> GSDQPRPTVIITGASSGVGLYATK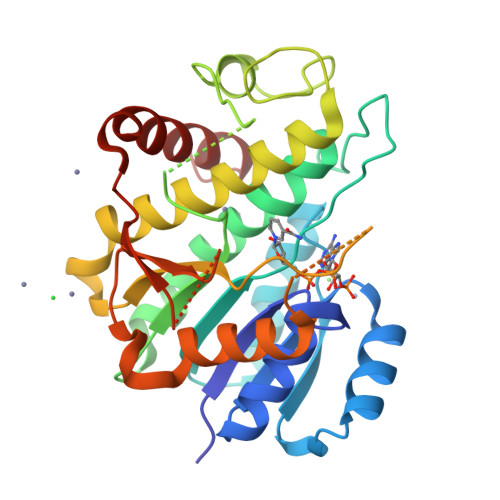ALANRGWHVIMACRNLEKAEQAAKNLQIPPEAYTILHLDLSSLASVRGFVESFRALNRPLRALVCNAAVYYPLLKEPIYSVDGYEITVATNHLGHFLLINLLLEDLKNSPESDKRLVILGTVTANRKELGGKIPIPAPPDLGNLEGFEKGFKKPIAMINGKPFKSGKAFKDSKLCNMLTARELHRRFHESTGIVFNSLYPGCVADTPLFRHHFPLFQKLFPLFQKKITGGYVSQELAGERVAMVVADPEFRQSGVHWSWGNRQKEGRKAFVQELSAEASDEQKARRLWELSEKLVGLA> MPASRYITDMTIEELSRDWFMLMPKQKVEGPLCIRIDQAIMDKNIMLKANFSVIFDRLETLILLRA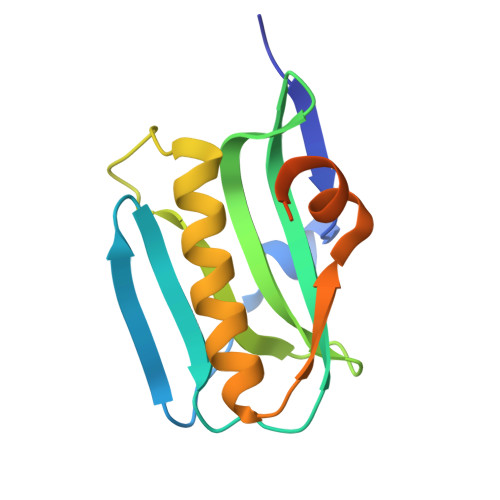FTEEGAIVGEISPLPSFPGHTIEDVKNAIGVLIGGLEWNDNTVRVSKTLQRFAWGSSNENGRPPLTLEHHHHHH2-[[2-fluoro-5-[[[4-[(Z)-(4-oxo-2-sulfanylidene-1,3-thiazolidin-5-ylidene)methyl]phenyl]amino]methyl]phenyl]carbonylamino]pentanedioic 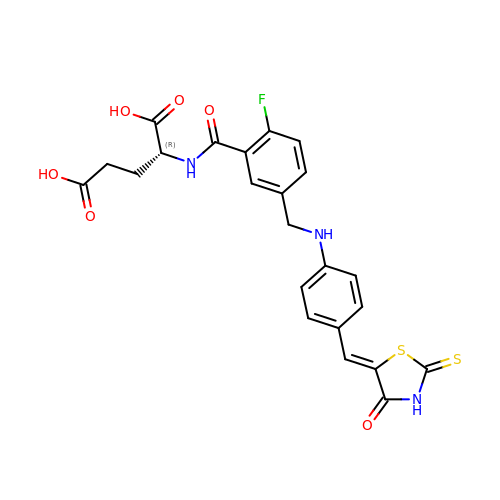acid | C23 H20 F N3 O6 S2 | NEGUDZMAJDITEM-RMFUMNGISA-N>[2x]SQIGLFSKICRVTIKTLHYYNKIGLLVPAYINPDNGYRFYTSDQLMKFHQIASLRQLGFTITEIVTLTQDENSCHIIERRRLEIQKQIRDMADMLSRINHYLQHKKKERIMLYQAALKEIPECIVYSKRFIVPDFSSYIKLIPPIGQEVMKANPGLTLTTPAYCFTLYHDKEYKEKNMDVEFCEAVNDFGKNEGNI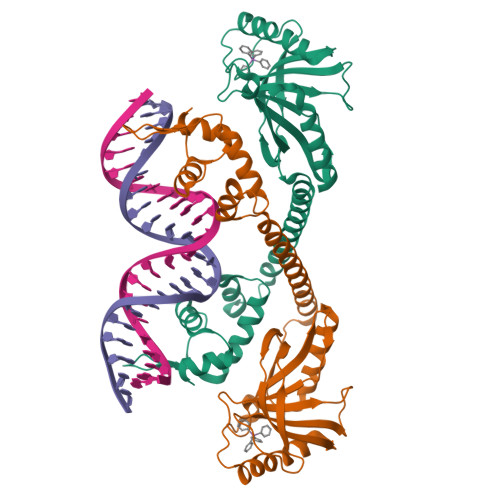IFQVIPAITAVTVIHKGPYDSLRNAYIYLMQWVEDNGYLLTNSPRESYIDGIWNKQDSAEWMTEIQFPVEKV>[9x]QLHQQQHQ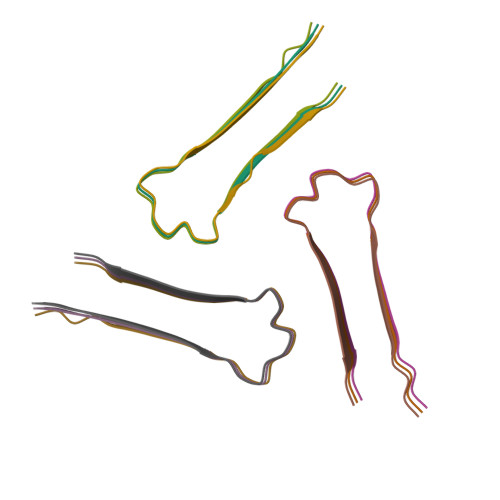QQHQQHQQHQQQQQLHQHQQQLS>[6x]PIELLPETPSQTAGPYVHIGLALEAAGNPTRDQEIWNRLAKPDAPGEHILLLGQVYDGNGHLVRDSFLEVWQADANGEYQDAYNLENAFNSFGRT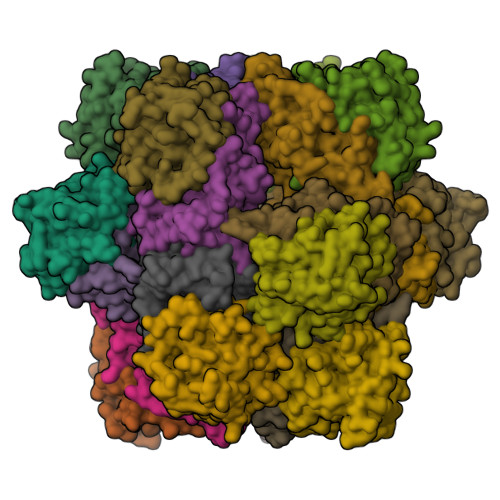ATTFDAGEWTLHTVKPGVVNNAAGVPMAPHINISLFARGINIHLHTRLYFDDEAQANAKCPVLNLIEQPQRRETLIAKRCEVDGKTAYRFDIRIQGEGETVFFDF;>PAQDNSRFVIRDRNWHPKALTPDYKTSIARSPRQALVSIPQSISETTGPNFSHLGFGAHDHDLLLNFNNGGLPIGERIIVAGRVVDQYGKPVPNTLVEMWQANAGGRERHKNDRYLAPLDPNFGGVGRCLTDSDGYYSFRTIKPGPYPWRNGPNDWRPAHIHFGISGPSIATKLITQLYFEGDPLIPMCPIVKSIANPEAVQQLIAKLDMNNANPMDCLAYRFDIVLRGQRKTHFENC[6x]(3P)-4-[4-(hydroxymethyl)phenyl]-3-(2H-tetrazol-5-yl)pyridine-2-sulfonamide | C13 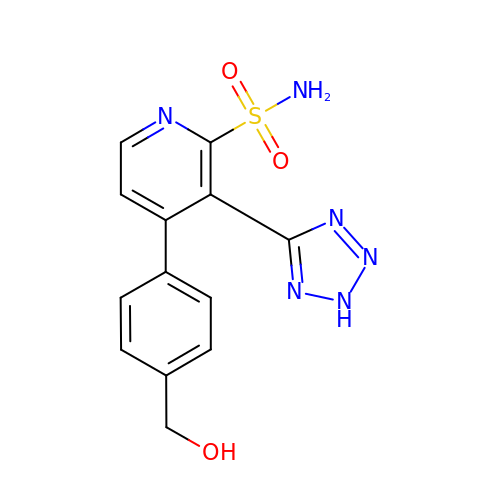H12 N6 O3 S | ZLLPEJMJTQBWDI-UHFFFAOYSA-N>[3x]MGIGKSPTGIQGFDELTLGGLPTGRPSLVCGSAGCGKTLFASTFLINGVRDHGEPGVFVTFEERPEDIVNNVASLGFELDKLIEEEKIAIEHIAVDPSEVAEIGDYDLEGLFLRLELAIDTVGAKRVVLDTIESLFSAFSNPAILRAEIRRLFDWLKERGLTTVITAERGDGALTRQGLEEYVSDCVILLDHRVEN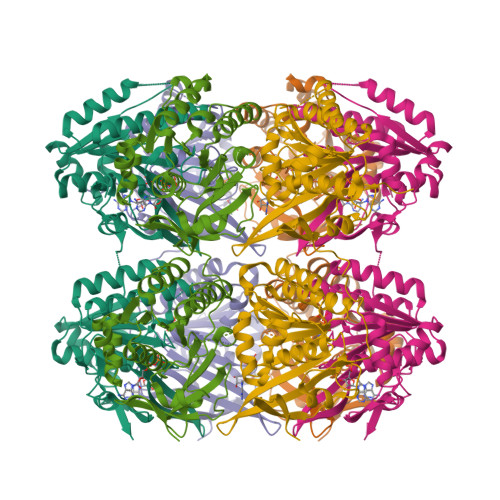QISTRRLRIVKYRGTAHGTNEYPFLIDTDGFSVLPVSALGLLHQVHEERIASGVPDLDAMMAGGGFFRGSSILVSGVAGAGKSSLAAHFAAAACARGERAMYFSFEEAADQAVRNMRSLGLDLGRWRDAGLLRFMATRPTFYSLEMHLAVILREVMRFEPSVVVLDPISAFTESGDRLEVQSMLLRIVDFLKNRGITGIFTHLAHSQNEATTDAGLSSLMDGWVLMLNREVNGEFNRELYLLKARGMAHSNQVREFLMSDRGISLLPPHLGEGGALTGTARKAEEARLRRAEIE> GCGCGGAUAGCUCAGUCG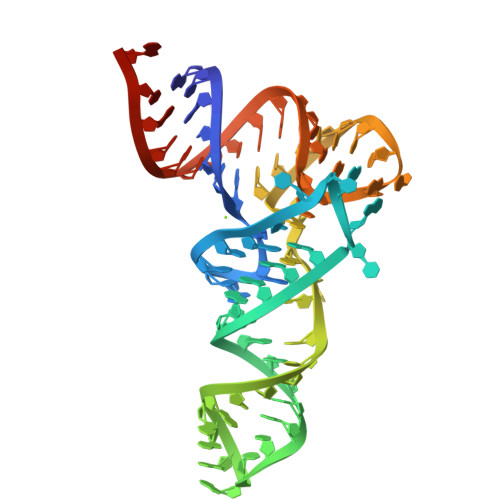GUAGAGCAGGGGAUUGAAAAUCCCCGUGUCCUUGGUUCGAUUCCGAGUCCGCGCACCA Here we present a series of TIGR03971 SDR crystal structures from several mycobacterial species which contain an insertion in the primary sequence at the NAD cofactor binding site. These crystal structures demonstrate that the inserted protein residues almost completely cover the NAD cofactor, only leaving part of the nicotinamide ring exposed to solvent. NMR experiments did not show exchange of the NAD cofactor, whereas binding was demonstrated for a number of small molecules which could be potential substrates, products, inhibitors, or artificial redox partners. Experimental results are consistent with the notion that the SDR family enzymes linked by comparative genomics studies to mycofactocin do indeed keep their NAD tightly bound beneath a protein structure that may interact with a specialized adaptor machinery for redox exchange.

With the exception of the M. thermoresistibile target which did not contain NAD, all other mycobacterial SDR target crystal structures contained NAD, which appears to have co-purified with the protein after expression in E. coli. For each of these crystal structures, the adenosine mononucleotide portion of the cofactor binding site is enveloped by the inserted residues and only a portion of the nicotinamide ring appears open to solvent (see representative examples in Fig. 2A and B). In addition to the insertion loop which covers the adenosine portion of the cofactor, a second loop which typically contains two α-helices covers much of nicotinamide mononucleotide portion of the cofactor. In contrast, this loop is ordered in each of the mycobacterial SDR crystal structures presented here. The combination of the insertion loop which covers the adenosine portion of the cofactor and the ordering of the second loop which covers the nicotinamide mononucleotide portion of the cofactor results in a significant decrease in the solvent accessible surface area of the cofactor in the mycobacterial SDRs, relative to other NAD- and NADP-dependent dehydrogenases. Only a small portion of the nicotinamide ring appears available to solvent in each of these cases, indicating that the NAD cofactor is tightly bound and potentially non-exchangeable. The structures presented here have a cofactor solvent accessible surface area of approximately 18 Å2, whereas other NAD- or NADP-bound dehydrogenases have a cofactor solvent accessible surface area of 82–89 Å2. Given the encapsulation of the NAD cofactor by the two loops in mycobacterial SDRs, a large conformational change would be required to release the NADH cofactor after a redox reaction had occurred. Alternatively, these structural elements may not allow for exchange of bound NAD/NADH with free NAD/NADH.

>[4x]GPGSMAGKLEGRVAFITGAARGQGRAHAVRMAAEGADIIAVDIAGKLPSCVPYDPASPDDLSETVRLVEAANRRIVAAVVDTRDFDRLRKVVDDGVAALGRLDIIVANAGVAAPQAWDDITPEDFRDVMDINVTGTWNTVMAGAPRIIEGGRGGSIILISSAAGMKMQPFMIHYTASKHAVTGLARAFAAELGKHSIRVNSVHPGPVNTPMGSGDMVTAVGQAMETNPQLSHVLTPFLPDWVAEPEDIADTVCWLASDESRKVTAAQIPVDQGSTQY2-HYDROXYCYCLOHEPTA-2,4,6-TRIEN-1-ONE | C7 H6 O2 | 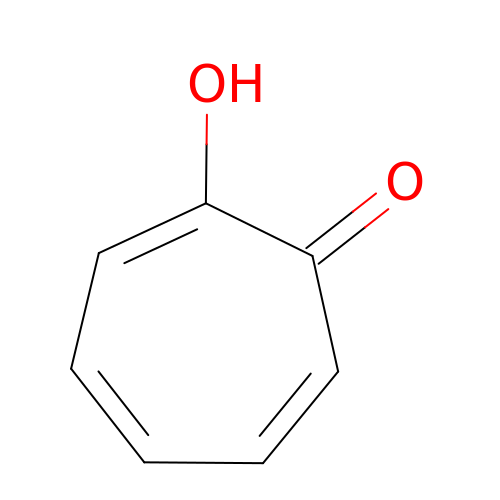MDYOLVRUBBJPFM-UHFFFAOYSA-N>[2x]GSDWVIPPINLPENS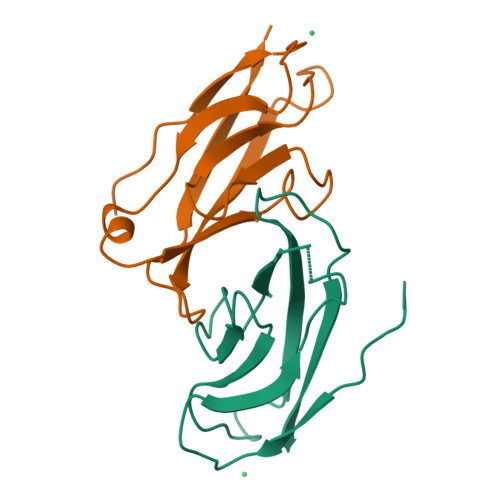RGPFPQELVRIRSGRDKNLSLRYSVTGPGADQPPTGIFIINPISGQLSVTKPLDRELIARFHLRAHAVDINGNQVENPIDIVINVIDMNDNRPEF>MASMTGGQQMGRDEAGITGTWYNQLGSTFIVTAGADGALTGTYESAAGKA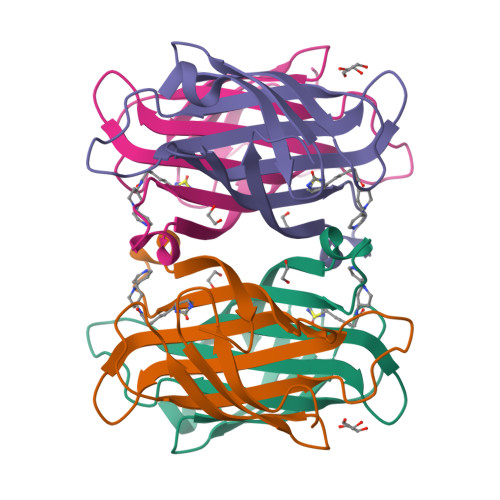ESRYVLTGRYDSAPATDGSGTALGWTVAWKNNYRNAHSATTWSGQYVGGAEARINTQWLLTAGATEANGWASTYVGHDTFTKVKPSAASIDAAKKAGVNNGNPLDAVQQ[2x]> MGRKKIQISRILDQRNRQVTFTKRKFGLMKKAYELSVLCDCEIALIIFN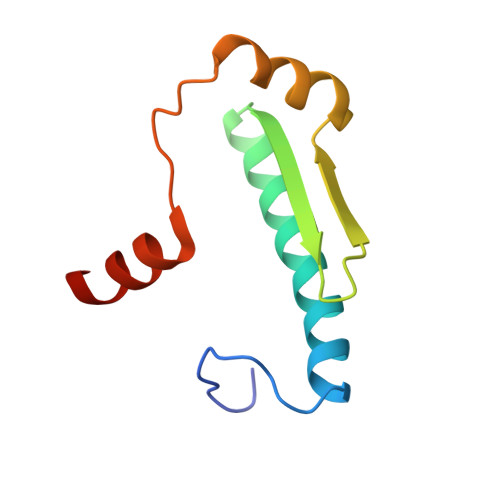SANRLFQYASTDMDRVLLKYTEYSEPHESRTNTDILETLKRRGI> YRAFDIYNDKVAGFAKFLKTNCCRFQEKDEDDNLIDSYFVVKRHTFSNYQHEETIYNLLKDCPAVAKHDFFKFRIDGDMVPHISRQRLTKYTMADLVYALRHFDEGNCDTLKEILVTYNCCDDDYFNKKDWYDFVENPDILRVYANLGERVRQALLKTVQFCDAMRNAGIVGVLTLDNQDLNGNWYDFGDFIQTTPGSGVPVVDSYYSLLMPILTLTRALTAESHVDTDLTKPYIKWDLLKYDFTEERLKLFDRYFKYWDQTYHPNCVNCLDDRCILHCANFNVLFSTVFPPTSFGPLVRKIFVDGVPFVVSTGYHFRELGVVHNQDVNLHSSRLSFKELLVYAADPAMHAASGNLLLDKRTTCFSVAALTNNVAFQTVKPGNFNKDFYDFAVSKGFFKEGSSVELKHFFFAQDGNAAISDYDYYRYNLPTMCDIRQLLFVVEVVDKYFDCYDGGCINANQVIVNNLDKSAGFPFNKWGKARLYYDSMSYEDQDALFAYTKRNVIPTIT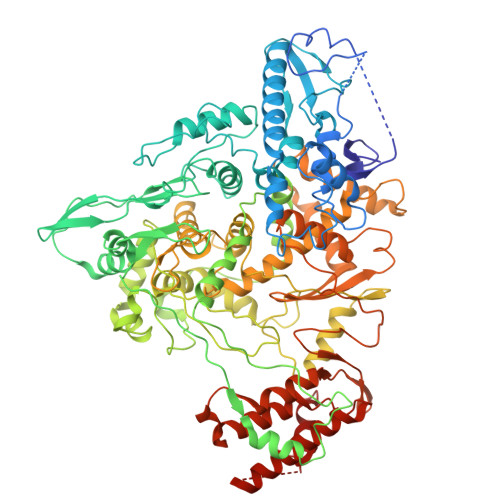QMNLKYAISAKNRARTVAGVSICSTMTNRQFHQKLLKSIAATRGATVVIGTSKFYGGWHNMLKTVYSDVENPHLMGWDYPKCDRAMPNMLRIMASLVLARKHTTCCSLSHRFYRLANECAQVLSEMVMCGGSLYVKPGGTSSGDATTAYANSVFNICQAVTANVNALLSTDGNKIADKYVRNLQHRLYECLYRNRDVDTDFVNEFYAYLRKHFSMMILSDDAVVCFNSTYASQGLVASIKNFKSVLYYQNNVFMSEAKCWTETDLTKGPHEFCSQHTMLVKQGDDYVYLPYPDPSRILGAGCFVDDIVKTDGTLMIERFVSLAIDAYPLTKHPNQEYADVFHLYLQYIRKLHDELTGHMLDMYSVMLTNDNTSRYWEPEFYEAMYTPHT>MNEQIPHDKSLDNSLTLLKEGYLFIKNRTERYNSDLFQARLLGKNFICMTGAEAAKVFYDTDRFQRQNALPKRVQKSLFGVNAIQGMDGSAHIHRKMLFLSLMTPPHQKRLAELMTEEWKAAVTRWEKADEVVLFEEAKEILCRVACYWAGVPLKETEVKERADDFIDMVDAFGAVGPRHWKGRRARPRAEEWIEVMIEDARAGLLKTTSGTALHEMAFHTQEDGSQLDSRMAAIELINVLRPIVAISYFLVFSALALHEHPKYKEWLRSGNSREREMFVQEVRRYYPFGPFLGALVKKDFVWNNCEFKKGTSVLLDLYGTNHDPRLWDHPDEFRPERFAEREENLFDMI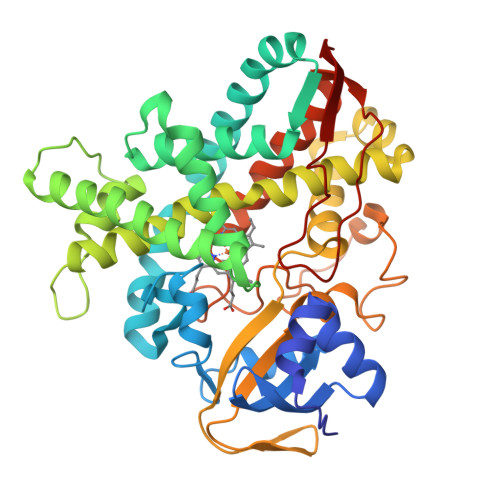PQGGGHAEKGHRCPGEGITIEVMKASLDFLVHQIEYDVPEQSLHYSLARMPSLPESGFVMSGIRRKS[3x]> MASSRRESINPWILTGFADAEGSFGLSILNRNRGTARYHTRLSFTIMLHNKDKSILENIQSTWKVGSILNNGDHYVSLVVYRFEDLKVIIDHFEKYPLITQKLGDYKLFKQAFSVMENKEHLKENGIKELVRIKAKMN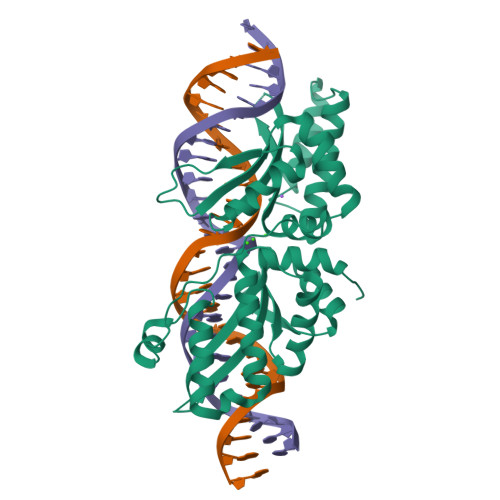WGLNDELKKAFPENISKERPLINKNIPNFKWLAGFTSGDGSFFVRLRKSNVNARVRVQLVFEISQHIRDKNLMNSLITYLGCGHIYEGNKSERSWLQFRVEKFSDINDKIIPVFQENTLIGVKLEDFEDWCKVAKLIEEKKHLTESGLDEIKKIKLNMNKGR>[2x]DSMYGFIGTDVVLHCSFANPLPGVKITQVTWQKATNGSKQNVAIYNPAMGVSVLAPYRERVEFLRPSFTDGTIRLSRLELEDEGVYICEFATFPAGNRESQLNLTVMAK;>ADEFLPTPAPRVTVYVDPPAYPMPRYNYTERWHTTGPIPSPFADGREQPVEVRYATSAAACDMLALIADPQVGRTLWEAVRRHARAYNATVIWYKIESGCARPLYYMEYTECEPRKHFGY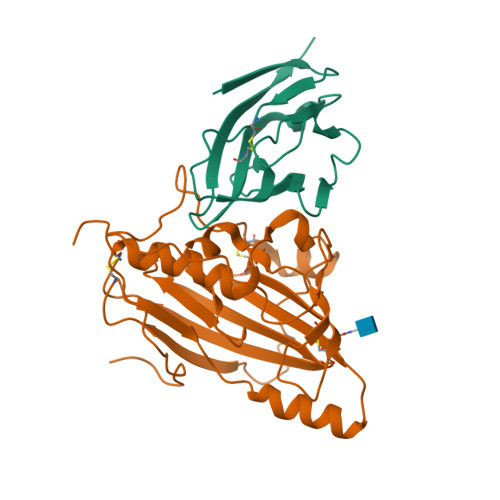CRYRTPPFWDSFLAGFAYPTDDELGLIMAAPARLVEGQYRRALYIDGTVAYTDFMVSLPAGDCWFSKLGAARGYTFGACFPARDYEQKKVLRLTYLTQYYPQEAHKAIVDYWFMRHGGVVPPYFEESKGYEPPPAADGGSPAPPGDDEAREDEGETEDGAAGREGNGGPPGPEGDGESQTPEANGHHHHHH[2x]>SNANDTDGDTLDVLLPLRTTGEKAPLFCVHPAGGLSWVYSGLMQHIGADRPLYGLQA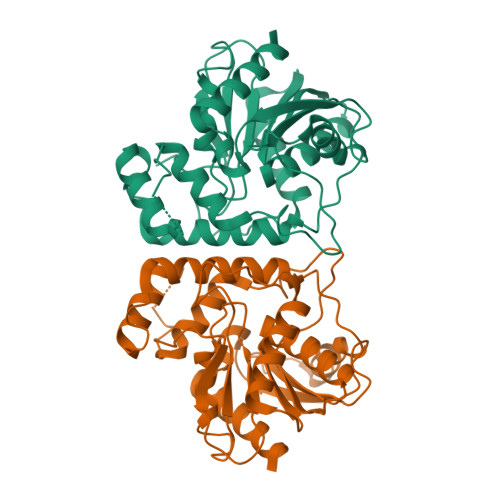RGLADPSATLPSSIEEMAADYVTQIRGVQPSGPYHLLGWALGSLVIHAMATQLRAEGEEVGLLVNLDQYPIDRSRPAPESQPDQQDALRIMLDFVGYDMDSLGDEPLDYAMVADVLRERQSVFANLDETAITALANVFANSRSLFGSFAPQPLDSDVLVIVAEPDETVPAAELAARVEQWRPFVTGKIEYQTVRCSHPHMMQPEPAAEIGRLIAEKLGTSK[3x]> GSKEGEYIKLKVIGQDSSEIHFKVKMTTHLKKL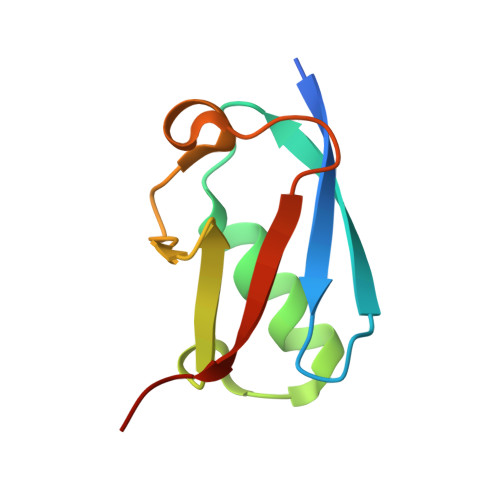KESYAQRQGVPMNSLRFLFEGQRIADNHTPKELGMEEEDVIEVYQEQTGG> MSPLSGSLAPLNMKGLVKFQDVSFAYPNHPNVQVLQGLTFTLYPGKVTALVGPNGSGKSTVAALLQNL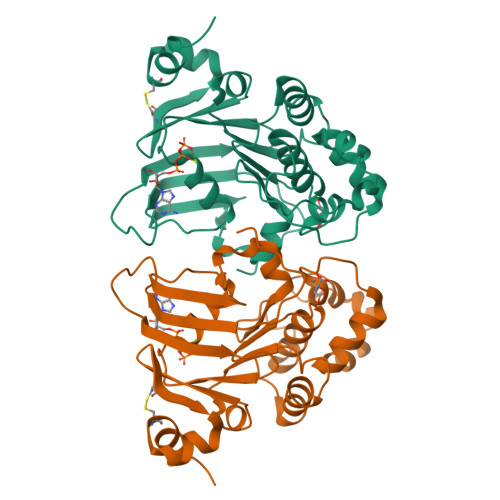YQPTGGKVLLDGEPLVQYDHHYLHTQVAAVGQEPLLFGRSFRENIAYGLTRTPTMEEITAVAMESGAHDFISGFPQGYDTEVGETGNQLSGGQRQAVALARALIRKPRLLILDNATSALAAGNQLRVQRLLYESPEWASRTVLLITQQLSLAERAHHILFLKEGSVCEQGTHLQLMERGGCYRSMVEALAAPSDAAAHHHHHH> AAAAALSTLSSTESLTISSNRTLVSPGNIFELGFFRTNSRWYLGMWYKKLSGRTYVWVANRDNPLSNSIGTLKISNMNLVLLDHSNKSVWSTNLTRENVRSPVVAELLANGNFVVRDPSGFLWQSFDYPTDTLLPEMKLGYDLKTGLNRFLVSWRSS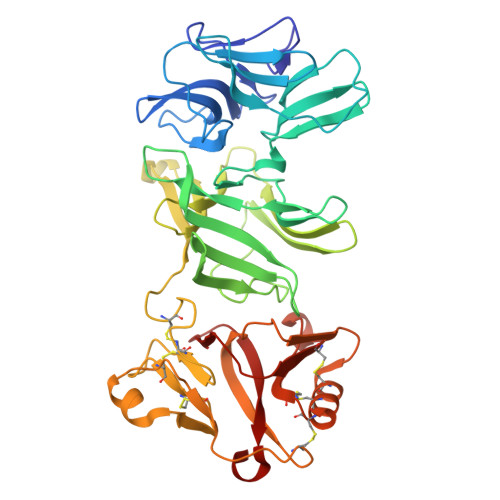DDPSSGDFSYKLDIQRGLPEFYTFKDNTLVHRTGPWNGIRFSGIPEEQQLSYMVYNFTENSEEVAYTFLVTNNSIYSRLTINFSGFFERLTWTPSLVIWNPIWSSPASFQCDPYMICGPGSYCDVNTLPLCNCIQGFKPLNVQEWDMRDHTRGCIRRTRLSCRGDGFTRMKNMKLPETTMATVDRSIGVKECEKKCLSDCNCTAFANADIRDGGTGCVIWTGRLDDMRNYAVSGQDLYVRLAAADVVE>[6x]MNDQTQFTERALTILTLAQKLASDHQHPQLQPIHILAAFIETPEDGSVPYLQNLIEKGRYDYDLFKKVVNRNLVRIPQQQPAPAEITPSYALGKVLQDAAKIQKQQKDSFIAQDHILFALFNDSSIQQIFKEAQVDIEAIKQQALELRGNTRIDS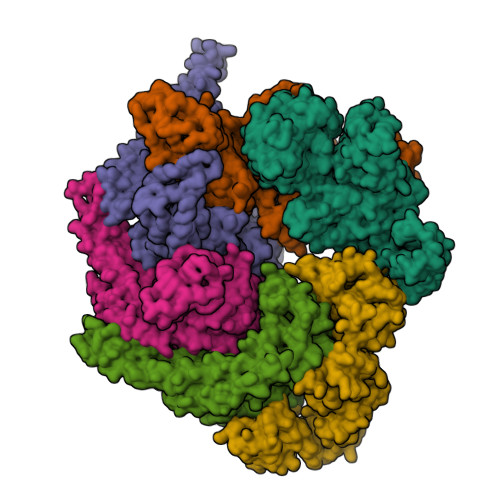RGADTNTPLEYLSKYAIDMTEQARQGKLDPVIGREEEIRSTIRVLARRIKSNPCLIGEPGIGKTAIIEGVAQRIIDDDVPTILQGAKLFSLDLAALTAGAKYKGDFEERFKGVLKEIEESKTLIVLFIDEIHMLMGNGKDDAANILKPALSRGQLKVIGATTNNEYRSIVEKDGAFERRFQKIEVAEPSVRQTVAILRGLQPKYEIHHGVRILDSALVTAAQLAKRYLPYRRLPDSALDLVDISCAGVAVARDSKPEELDSKERQLQLIQVEIKALERDEDADSTTKDRLKLARQKEASLQEELEPLRQRYNEEKHGHEELTQAKKKLDELENKALDAERRYDTATAADLRYFAIPDIKKQIEKLEDQVAEEERRAGANSMIQNVVDSDTISETAARLTGIPVKKLSESENEKLIHMERDLSSEVVGQMDAIKAVSNAVRLSRSGLANPRQPASFLFLGLSGSGKTELAKKVAGFLFNDEDMMIRVDCSELSEKYAVSKLLGTTAGYVGYDEGGFLTNQLQYKPYSVLLFDEVEKAHPDVLTVMLQMLDDGRITSGQGKTIDCSNCIVIMTSALGAEFINSQQGSKIQESTKNLVMGAVRQHFRPEFLNRISSIVIFNKLSRKAIHKIVDIRLKEIEERFEQNDKHYKLNLTQEAKDFLAKYGYSDDMGARPLNRLIQNEILNKLALRILKNEIKDKETVNVVLKKGKSRDENVPEEAEECLEVLPNHEATIGADTLGDDDNEDSMEIDDDLD> MERTELLKPRTLADLIRILHELFAGDEVNVEEVQAVLEAYESNPAEWALYAKFDQY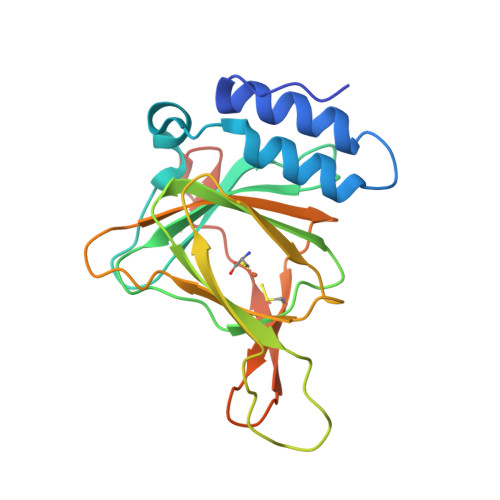RYTRNLVDQGNGKFNLMILCWGEGHGSSIHDHTDSHCFLKLLQGNLKETLFDWPDKKSNEMIKKSERTLRENQCAYINDSIGLHRVENVSHTEPAVSLHLYSPPFDTCHAFDQRTGHKNKVTMTFHSKFGIRTPFTTSGSLENN> MQDAITAVINASDVQGKYLDTAAME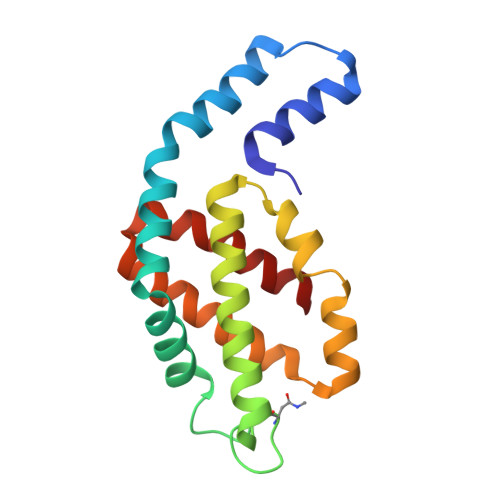KLKAYFATGELRVRAASVISANAANIVKEAVAKSLLYSDITRPGGNMYTTRRYAACIRDLDYYLRYATYAMLAGDPSILDERVLNGLKETYNSLGVPIAATVQAIQAMKEVTASLVGADAGKEMGIYFDYICSGLS> GPLGSPFQCSLCSYASRDTYKLKRHMRTHSGEKPYECYICHARFTQSGTMKMHILQKHT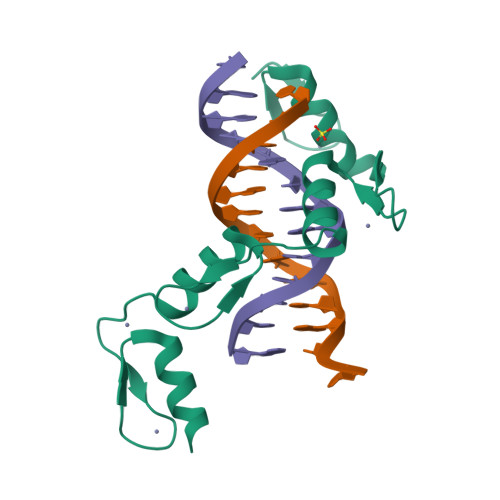ENVAKFHCPHCDTVIARKSDLGVHLRKQHSYIEQGKKCRYCDAVFHERYALIQHQKSH~{N}-[2-[[6-chloranyl-3-[3-[4-(hydroxymethyl)piperidin-1-yl]sulfonyl-4-methoxy-phenyl]-2-methyl-imidazo[1,2-b]pyridazin-8-yl]amino]ethyl]ethanamide 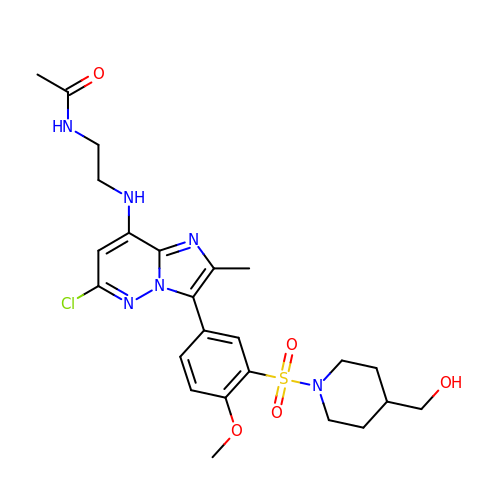| C24 H31 Cl N6 O5 S | IEPPNMCWFCTFFK-UHFFFAOYSA-N N-ALPHA-(2-NAPHTHYLSULFONYL)-N-(3-AMIDINO-L-PHENYLALANINYL)-D-PIPECOLINIC ACID | C26 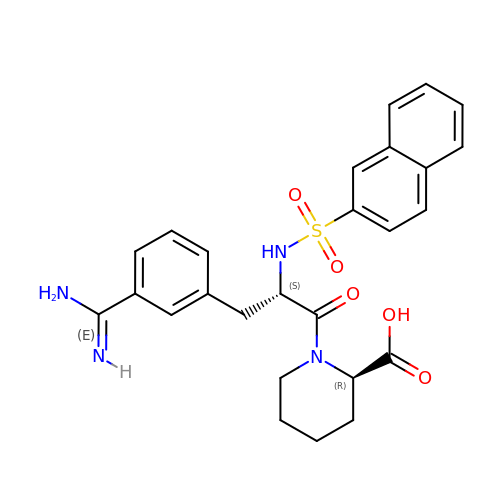H28 N4 O5 S | GNANSBQAIRJZPA-XZOQPEGZSA-N>[2x]MSTVTTINLEDIKEIMHTTIRLGGKPESGEAAELPIFLGSSVEFEAELYDADGTQIGTAKGTSVIFAEADGTVMQIVSAFDDYTDGGRVTWSGAYTMFPTD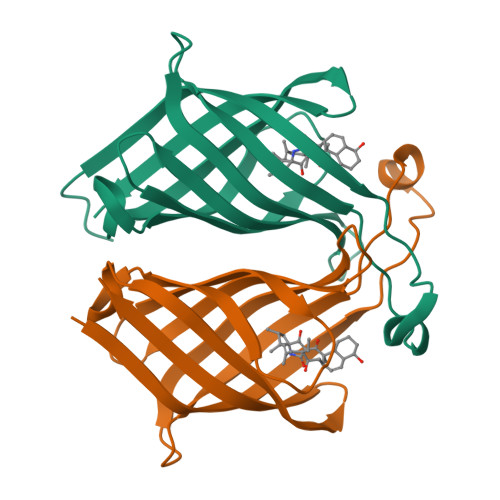EPKSVPAQGVSGRYRGLSGTRTFQLLERPDPGTSLVRSSLVLNG>XXXXXXXXXXXXXXXXXXXXXXXXXXXXXXXXXXXXXXXXXXXXXXXXXXXXXXXXXXXXXXXXXXXXXXXXXXXXXXXXXXXXXXXXXXXXXXXXXXXXXXXXXXXXXXXXXXXXXXXXXKFLTIPRLEELYNTKQGPTNPMLFHLIRDVKQGNLPPGYKITLIDIGLVIEYLMGGTYRCTYTRKRFRLIYNSLGGNNRRSGRNTSSSTPQLRKSHETFGNRADKKEKMRHNHFIKTAQPYRPKMDASMEEGKKKRTKDEIVDIDDPETKRFPYPLNELLIWACLMKRQVMARFLWQHGEESMAKALVACKIYRSMAYEAKQSDLVDDTSEELKQYSNDFGQLAVELLEQSFRQDETMAMKLLTYELKNWSNSTCLKLAVSSRLRPFVAHTCTQMLLSDMWMGRLNMRKNSWYKVILSILVPPAILMLEYKTKAEMSHIPQSQDAHQMTMEDSENNFHNITEEIPMEVFKEVKILDSSDGKNEMEIHIKSKKLPITRKFYAFYHAPIVKFWFNTLAYLGFLMLYTFVVLVKMEQLPSVQEWIVIAYIFTYAIEKVREVFMSEAGKISQKIKVWFSDYFNVSDTIAIISFFVGFGLRFGAKWNYINAYDNHVFVAGRLIYCLNIIFWYVRLLDFLAVNQQAGPYVMMIGKMVANMFYIVVIMALVLLSFGVPRKAILYPHEEPSWSLAKDIVFHPYWMIFGEVYAYEIDVCANDSTLPTICGPGTWLTPFLQAVYLFVQYIIMVNLLIAFFNNVYLQVKAISNIVWKYQRYHFIMAYHEKPVLPPPLIILSHIVSLFCCVCKRRKKDKTSDGPKLFLTEEDQKKLHDFEEQCVEMYFDEKDDKFNSGSEERIRVTFERVEQMSIQIKEVGDRVNYIKRSLQSLDSQIGHLQDLSALTVDTLKTLTAQKASEASKVHNEITRELSISK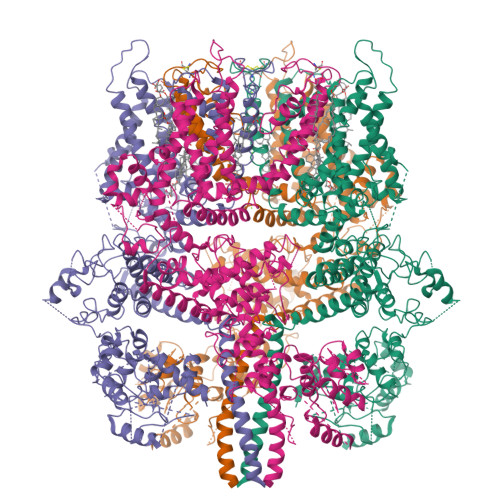HLAQNLIDDVPVRPLWKKPSAVNTLSSS[4x]> SMFLPPPECPVFEPSWEEFADPFAFIHKIRPIAEQTGICKVRPPPDWQPPFACDVDKLHFTPRIQRLNELEAQTRVKLGGGGGFEQAARDYTLRTFGEMADAFKSDYFNMPVHMVPTELVEKEFWRLVSTIEEDVTVEYGADIASKEFGSGFPVRDGKIKLSPEEEEYLDSGWNLNNMPVMEQSVLAHITADICGMKLPWLYVGMCFSSFCWHIEDHWSYSINYLHWGEPKTWYGVPGYAAEQLENVMKKLAPELFVSQPDLLHQLVTIMNPNTLMTHEVPVYRTNQCAGEFVITFPRAYHSGFNQGFNFAEAVNFCTVDWLPLGRQCVEHYRLLHRYCVFSHDEMICKMASKADVLDVVVASTVQKDMAIMIEDEKALRETVRKLGVIDSERMDFELLPDDERQCVKCKTTCFMSAISCSCKPG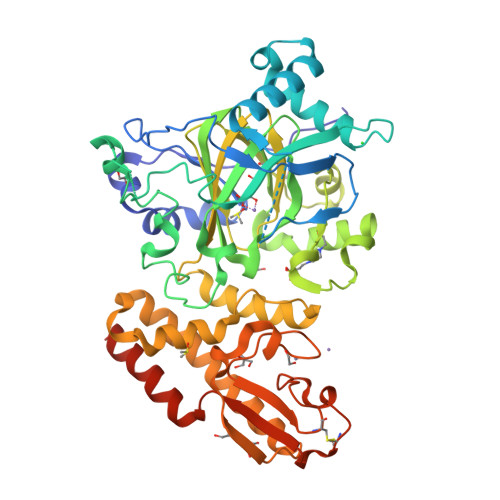LLVCLHHVKELCSCPPYKYKLRYRYTLDDLYPMMNALKLRAESYNEWALNVNEALEAKI>[2x]MSLKDFAGRTAFVTGGA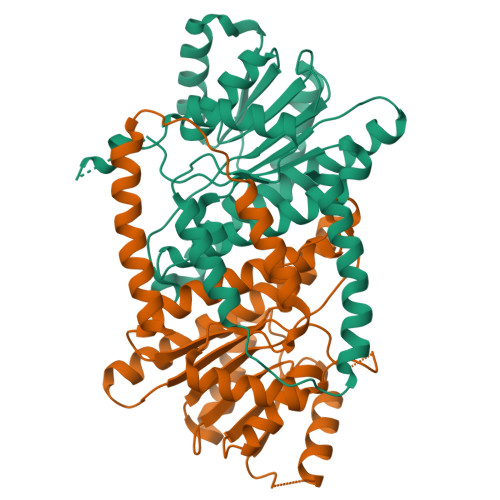NGVGIGLVRQLLNQGCKVAIADIRQDSIDKALATLEAEGSGPEVMGVQLDVASREGFKMAADEVEARFGPVSILCNNAGVNLFQPIEESSYDDWDWLLGVNLHGVVNGVTTFVPRMVERVKAGEQKGGHVVNTASMAAFLAAGSPGIYNTTKFAVRGLSESLHYSLLKYEIGVSVLCPGLVKSYIYASDDIRPDALKGEVKPVDKTAVERLAGVHEFGMEPDVIGARVIEAMKANRLHIFSHPDHKEELREVFDEIIAEYQDYPKDPGYDQRVAFEKFRADSFAEARRQSRAADEGHHHHHH>MARRLPKPTLQGRLEADFPDSPLLPKFQELNQNNLPNDVFREAQRSYLVFLTSQFCYEEYVQRTFGVPRRQRAIDKRQRASVAGAGAHAHLGGSSATPVQQAQAAASAGTGALASSAPSTAVAQSATPSVSSSISSLRAATSGATAAASAAAAVDTGSGGGGQPHDTAPRGARKKQ[5x];>MKVQGSVDRRRLQRRIAGLLPPPARRLNISRGSEFTRDVRGLVEEHAQASSLSAAAVWRAGLLAPGEVAVAGGGSGGGSFSWSGWRPPVFGDFLIHASSFNNAEATGTPLFQFKQSDPFSGVDAVFTPLSLFILMNHGRGVAARVEAGGGLTRMANLLYDSPATLADLVPDFGRLVADRRFHNFITPVGPLVENIKSTYLNKITTVVHGPVVSKAIPRSTVKVTVPQEAFVDLDAWLSGGAGGGGGVCFVGGLGLQPCPADARLYVALTYEEAGPRFTFFQSSRGHCQIMNILRIYYSPSIMHRYAVVQPLHIEELTFGAVACLGTFSATDGWRRSAFNYRGSSLPVVEIDSFYSNVSDWEVIL[2x];>[4x]MDLKVVVSLSSRLYTDEIAKMQQRIGCILPLASTHGTQNVQGLGLGQVYSLETVPDYVSMYNYLSDCTLAVLDEVSVDSLILTKIVPGQTYAIKNKYQPFFQWHGTGSLSVMPPVFGREHATVKLESNDVDIVFPMVLPTPIAEEVLQKILLFNVYSRVVMQAPGNADMLDVHMHLGSVSYLGHHYELALPEVPGPLGLALLDNLSLYFCIMVTLLPRASMRLVRGLIRHEHHDLLNLFQEMVPDEIARIDLDDLSVADDLSRMRVMMTYLQSLASLFNLGPRLATAAYSQETLTATCWLR;>[5x]MASNEGVENRPFPYLTVDADLLSNLRQSAAEGLFHSFDLLVGKDAREAGIKFEVLLGVYTNAIQYVRFLETALAVSCVNTEFKDLSRMTDGKIQFRISVPTIAHGDGRRPSKQR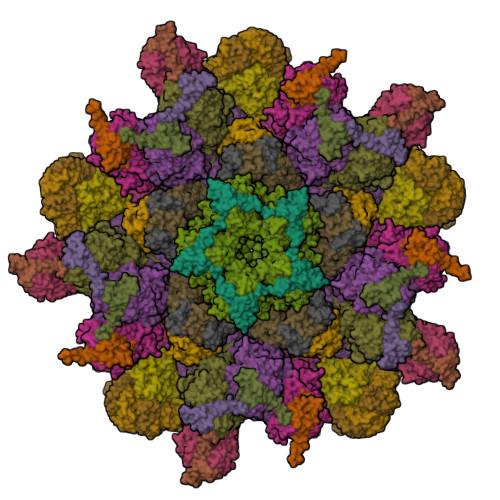TFIVVKNCHKHHISTEMELSMLDLEILHSIPETPVEYAEYVGAVKTVASALQFGVDALERGLINTVLSVKLRHAPPMFILQTLADPTFTERGFSKTVKSDLIAMFKRHLLEHSFFLDRAENMGSGFSQYVRSRLSEMVAAVSGESVLKGVSTYTTAKGGEPVGGVFIVTDNVLRQLLTFLGEEADNQIMGPSSYASFVVRGENLVTAVSYGRVMRTFEHFMARIVDSPEKAGSTKSDLPAVAAGVEDQPRVPISAAVIKLGNHAVAVESLQKMYNDTQSPYPLNRRMQYSYYFPVGLFMPNPKYTTSAAIKMLDNPTQQLPVEAWIVNKNNLLLAFNLQNALKVLCHPRLHTPAHTLNSLNAAPAPRDRRETYSLQHRRPNHMNVLVIVDEFYDNKYAAPVTDIALKCGLPTEDFLHPSNYDLLRLELHPLYDIYIGRDAGERARHRAVHRLMVGNLPTPLAPAAFQEARGQQFETATSLAHVVDQAVIETVQDTAYDTAYPAFFYVVEAMIHGFEEKFVMNVPLVSLCINTYWERSGRLAFVNSFSMIKFICRHLGNNAISKEAYSMYRKIYGELIALEQALMRLAGSDVVGDESVGQYVCALLDPNLLPPVAYTDIFTHLLTVSDRAPQIIIGNEVYADTLAAPQFIERVGNMDEMAAQFVALYGYRVNGDHDHDFRLHLGPYVDEGHADVLEKIFYYVFLPTCTNAHMCGLGVDFQHVAQTLAYNGPAFSHHFTRDEDILDNLENGTLRDLLEISDLRPTVGMIRDLSASFMTCPTFTRAVRVSVDNDVTQQLAPNPADKRTEQTVLVNGLVAFAFSERTRAVTQCLFHAIPFHMFYGDPRVAATMHQDVATFVMRNPQQRAVEAFNRPEQLFAEYREWHRSPMGKYAAECLPSLVSISGMTAMHIKMSPMAYIAQAKLKIHPGVAMTVVRTDEILSENILFSSRASTSMFIGTPNVSRREARVDAVTFEVHHEMASIDTGLSYSSTMTPARVAAITTDMGIHTQDFFSVFPAEAFGNQQVNDYIKAKVGAQRNGTLLRDPRTYLAGMTNVNGAPGLCHGQQATCEIIVTPVTADVAYFQKSNSPRGRAACVVSCENYNQEVAEGLIYDHSRPDAAYEYRSTVNPWASQLGSLGDIMYNSSYRQTAVPGLYSPCRAFFNKEELLRNNRGLYNMVNEYSQRLGGHPATSNTEVQFVVIAGTDVFLEQPCSFLQEAFPALSASSRALIDEFMSVKQTHAPIHYGHYIIEEVAPVRRILKFGNKVVF>SSWAAELAKPLTLDQLQQQNGKAIDTRPSAFYNGWPQTLNGPSGHELAALNLSASWLDKMSTEQLNAWIKQHNLKTDAPVALYGNDKDVDAVKTRLQKAGLTHISILSDALSEPSRLQKLPHFEQLVYPQWLHDLQQGKEVTAKPAGDWKVIEAAWGAPKLYLISHIPGADYIDTNEVESEPLWNKVS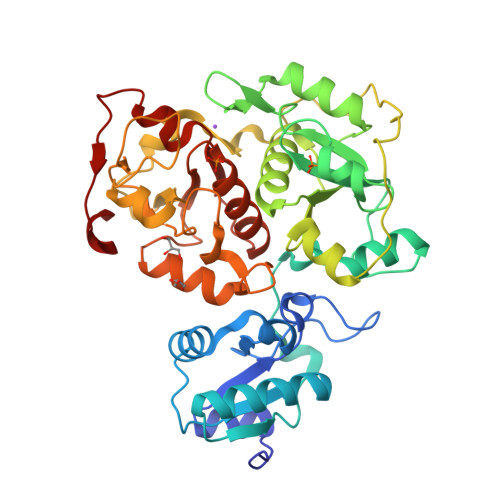DEQLKAMLAKHGIRHDTTVILYGRDVYAAARVAQIMLYAGVKDVRLLDGGWQTWSDAGLPVERGTPPKVKAEPDFGVKIPAQPQLMLDMEQARGLLHRQDASLVSIRSWPEFIGTTSGYSYIKPKGEIAGARWGHAGSDSTHMEDFHNPDGTMRSADDITAMWKAWNIKPEQQVSFYCGTGWRASETFMYARAMGWKNVSVYDGGWYEWSSDPKNPVATGERGPDSSK[2x]> DRRALRIGVNGLPPSLEPINGISNTGPRIINQIFDALIRRDYFADGAKGNNIKLVPALAESFERIDDKSIRFKLRQGVKFHNGAEMTAEDVAFTFSSERLWGDEAIKTVPNGRNFSPNWDEPVVEDKYTVVLRTKTPSYLIEKYLGSWLGPIVPKEYYKSLGAVAFGNKPIGTGPYKFRELVANDHVTLEANDGYWGDKPTASTITYQVVAEPATRVAGLISGEYDIITTLTPDDMALVDGYSDLETRGTLIENLHMFTFNMNQPIFQNKTLRRALALAVNRPLIVEALWKNKASIPNGFNFPHYGATYDPKRKPMEFNLKEAKRLVKESGYDGTPITYHTMGNYYANAVPALMMMIEMWKAAGITVVPKIFAPGTTPKDSDILIRNWSNGQWLTDGL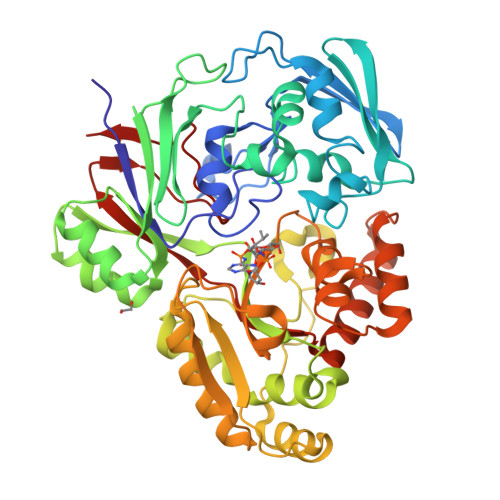TTMVSEFGPGRGVQKRWGWKAPAEFNNLCDQVAQLKDGEERSAAFNRLRDIFEDEAPAVLMYQPYDVYAARKDVQWSPVSFETMEFRGNLNFK> SVQPNFQQDKFLGRWFSAGLASNSSWLREKKAALSMAKSVVAPATDGGLNLTSTFLRKNQCETRTMLLQPAGSLGSYS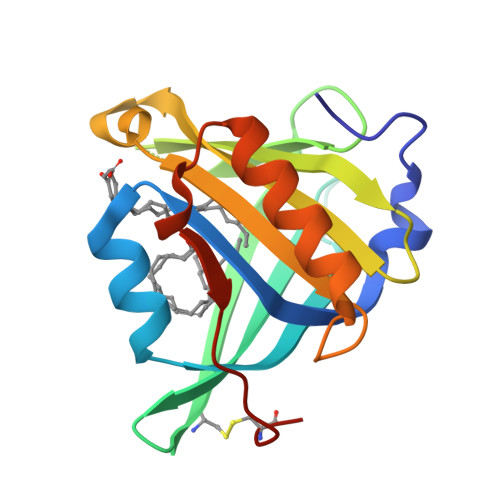YRSPHWGSTYSVSVVETDYDQYALLYSQGSKGPGEDFRMATLYSRTQTPRAELKEKFTAFCKAQGFTEDTIVFLPQTDKCMTEQ> MSSNRVLDLFKPFESFLPEVIAPERKVPYNQKLIWTGVSLLIFLILGQIPLYGIVSSETSDPLYWLRAMLASNRGTLLELGVSPIITSSMIFQFLQGTQLLQIRPESKQDRELFQIAQKVCAIILILGQALVVVMTGNYGAPSDLGLPICLLLIFQLMFASLIVMLLDELLSKGYGLGSGISLFTATNIAEQIFWRAFAPTTVNSGRGKEFEGAVIAFFHLLAVRKDKKRALVEAFYRTNLPNMFQVLMTVAIFLFVLYLQGFRYELPIRSTKVRGQIGIYPIKLFYTSNTPIMLQSALTSNIFLISQILFQKYPTNPLIRLIGVWGIRPGTQGPQMALSGLAYYIQPLMSLSEALLDPIKTIVYITFVLGSCAVFSKTWIEISGTSPRDIAKQFKDQGMVINGKRETSIYRELKKIIPTAAAFGGATIGALSVGSDLLGTLGSGASILMATTTIYGYYEAAAKEGGFTKNLVPGFSDLM;> MSSPTPPGGQRTLQKRKQGSSQKVAASAPKKNTNSNNSILKIYSDEATGLRVDPLVVLFLAVGFIFSVVALHVISKVAGKLF;> MARASEKGEEKKQSNNQVEKLVEAPVEFVREGTQFLAKCKKPDLKEYTKIVKAVGIGFIAVGIIGYAIKLIHIPIRYVIV;> GGSGGSGGSGGSGGSPTNYEYDEASETWPSFILTGLLMVVGPMTLLQIYQIFFGANAEDGNSGKSKEFNEEVFKNLNEEYTSDEIKQFRRKFDKNSNKKSKIWSRRNIIIIVGWILVAILLQRINSNDAIKDAATKLFDPYEILGISTSASDRDIKSAYRKLSVKFHPDKLAKGLTPDEKSVMEETYVQITKAYESLTDELVRQNYLKYGHPDGPQSTSHGIALPRFLVDGSASPLLVVCYVALLGLILPYFVSRWWARTQSYTKKGIHNVTASNFVSNLVNYKPSEIVTTDLILHWLSFAHEFKQFFPDLQPTDFEKLLQDHINRRDSGKLNNAKFRIVAKCHSLLHGLLDIACGFRNLDIALGAINTFKCIVQAVPLTPNCQILQLPNVDKEHFITKTGDIHTLGKLFTLEDAKIGEVLGIKDQAKLNETLRVASHIPNLKIIKADFLVPGRPYISLKVLVRSAKQPLIPTSLIPEENLTEPQDSESQRDPFA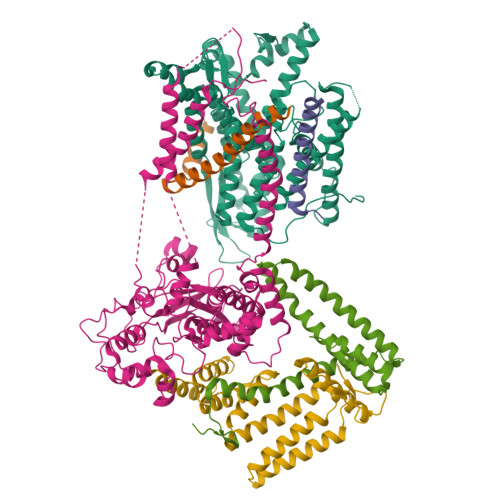MMSKQPLVPYSFAPFFPTKRRGSWCCLVSSQKDGKILQTPIIIEKLSYKNLNDDKDFFDKRIKMDLTKHEKFDINDWEIGTIKIPLGQPAPETVGDFFFRVIVKSTDYFTTDLDITMNMKVRDSPAVEQVEVYSEEDDEYSTDDDETESDDESDASDYTDIDTDTEAEDDESPEGENLYFQ;> MSEFNETKFSNNGTFFETEEPIVETKSISVYTPLIYVFILVVSLVMFASSYRKKQAKKISEQPSIFDENDAHDLYFQIKEMSENEKIHEKVLKAALLNRGAESVRRSLKLKELAPQINLLYKNGSIGEDYWKRFETEVKLIELEFKDTLQEAERLQPGWVQLFVMVCKEICFNQALSRRYQSILKRKEVCIKEWELKINNDGRLVN;> MVTLEYNANSKLITASDAVVALSTETNIDQINVLTTSLIGETNPNFTPQPNEALSKMIKGLFESGMKNLQQKKLNEALKNVSLAIEMAQRKRAPWEAFAIQLPELHFMLRSKIDLCLILGKHLEALQDLDFLLGTGLIQPDVFVRKADCLLKLRQWEEARATCERGLALAPEDMKLRALLIETARNLAEYNGE>[2x]MALLAEHLLKPLPADKQIETGPFLEAVSHLPPFFDCLGSPVFTPIKADISGNITKIKAVYDTNPAKFRTLQNILEVEKEMYGAEWPKVGATLALMWLKRGLRFIQVFLQSICDGERDENHPNLIRVNATKAYEMALKKYHGWIVQKIFQAALYAAPYKSDFLKALSKGQNVTEEECLEKIRLFLVNYTATIDVIYEMYTQMNAELNYKV

Human glycolipid transfer protein (hsGLTP) forms the prototypical GLTP fold and is characterized by a broad transfer selectivity for glycosphingolipids (GSLs). In human GLTP, a glycolipid headgroup recognition centre located on the protein surface enables selective binding of the GSL head and ceramide amide groups via multiple specific interactions. Encapsulation of lipid chains within the hydrophobic pocket involves a cleft-like gating mechanism that results in two glycolipid-binding modes. To elucidate the structural dynamics of the GLTP–GSL dimer and associated adaptations, we comparatively analyzed nine novel crystal structures of wild-type GLTP (wtGLTP) and the sulfatide-specific mutants D48V and A47D/D48V complexed with N-lauroyl-containing monosulfatide (N-lauroyl-3-O-sulfo-galactosylceramide; hereafter referred to as 12:0 monoSF) and disulfatide (N-lauroyl-3,6-di-O-sulfo-galactosylceramide; hereafter referred to as 12:0 diSF) in different crystal forms and compared them with previously studied GLTP–24:1 monoSF complexes.

To elucidate the dynamics of intermolecular interactions in the GLTP–disulfatide complex, we comparatively analyzed two crystal forms of wtGLTP and two crystal forms of the D48V mutant complexed with 12:0 diSF. The crystals of the wtGLTP–disulfatide complex represent ‘open’ and ‘closed’ conformations of the dimeric arrangement. However, adaptations within the open and closed dimers necessitate slightly different overall lipid conformations. The first noticeable deviations in the surface contact areas occur in wtGLTP–disulfatide complexes, which probably indicate a slightly different mutual orientation of monomers compared with wtGLTP–monosulfatide complexes. Interestingly, ligand adaptations also emerge with wtGLTP complexes bound with disulfatide. In contrast, the 6-O-sulfo group adopts different conformations/positions that depend on the protein (wild type or D48V) or the crystal type.> SVLVGCGNNTTNNNSGTSGPSTNSGTSGSGTNSGTTSNNVTGKTDLADTNFDTSYTPKRTSYKIYCTYKNIHAWYDAIKCGIDAAVKELAEKGVTVDYEWYG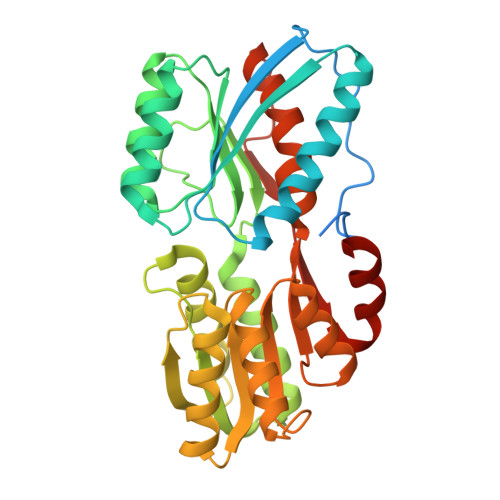PAQPDAVDQVNSIETAIGQGWDLIAVDVNQPELTGEAINNAVAKGIPVAVFGTSDVPNCDRAFFVGNTDPYGDGCALAKAVCEKMGGKGQIAILAGTIGALAHEERLRGFKDTIAKYPDIEIVDEQRDNDEVEKAISITESWLQAYPNLGGILCNNMSNPVGACQAVADAGKSGKIVIGGMDHDLRALNALKDGTLYVAQVQNCYDMGYKLIYNAIKTIDGEKVEESTAVGSTSVYAQDADKFINMLYGEAN> GSGAMTASELVAGDLAGGRAPGALPLDTTWHRPGWTIGELEAAKAGRTISVVLPALNEEATIESVIDSISPLVDGLVDELIVLDSGSTDDTEIRAIASGARVVSREQALPEVPVRPGKGEALWRSLAATSGDIVVFIDSDLINPHPLFVPWLVGPLLTGEGIQLVKSFYRRPLQVSDVTSGVCATGGGRVTELVARPLLAALRPELGCVLQPLSGEYAASRELLTSLPFAPGYGVEIGLLIDTFD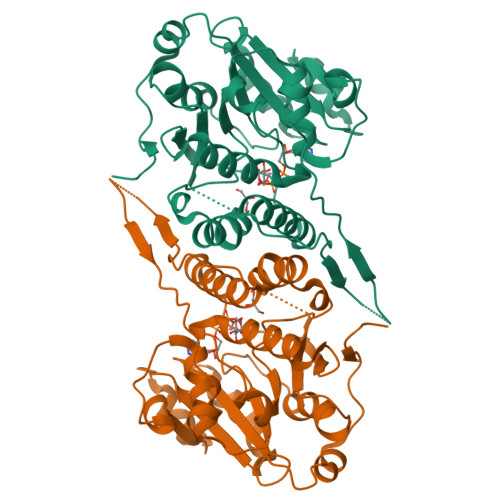RLGLDAIAQVNLGVRAHRNRPLDELGAMSRQVIATLLSRCGIPDSGVGLTQFLPGGPDDSDYTRHTWPVSLVDRPPMKVMRPR> QQQRCRHQFQTQQRLRACQRVIRRWSQGGGPMEDVEDEIDETDEIEEVVEPDQARRPPTLQRCCRQLRNVSPFCRCPSLRQAVQSAQQQQGQVGPQQVGHMYRVASRIPAIC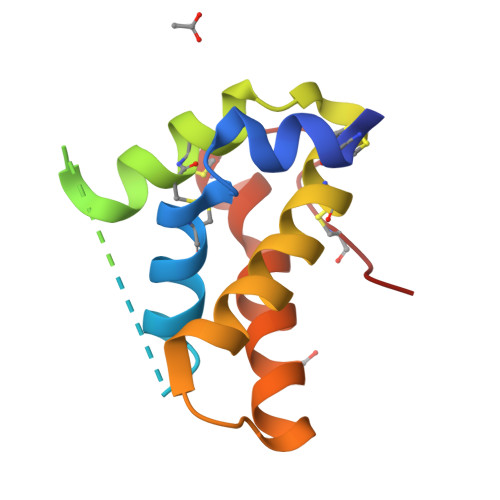NLQPMRCPFR>[2x]MGYLHRVVEGLKANAGGEALVSADRRLTGAETLEEIHRTARALAAQGLRPGDGVVTLHGNGVEAVVLRIAVQLLGCRYAGLRPVFATREKANFLAEAEAAAFVYQPDMADEAAELLREVPTPRVLSLGPAPLGEDLVALAGAQSAEPVEFTADERAATAVGFTGGTTGRAKGVCRAPFDLEACLDASLTIFGEGPWRFLVCIPIADLGGEMAEWTLAAGGTVVLREDFEPADILATIGAERTTHVFCAPGWVYQLAEHPALADADLSSLTQIPYGGAPSTPARIADALEKLGRPLLVHCYGSQEGGWMTWLSAEDHVRADRYLLNSVGKALPGTEIAIRDQDGADLPVGTVGEVCVRSTMLMRGYWRLPELTAKTVRDGWLHTGDLGRLDTEGYLYLVDRAKDVIIVEAYNVYSQEVEHVLTGHPDVRYAAVVGVPDHDTTEAVYAAVVPAEGVGEIDVDELRALVRTTLGPVHEPKHLDVVDTIPTTPRGHPDKSALRTRWRA

Amide Bond Synthetases (ABSs) actively catalyze both the ATP-dependent adenylation of carboxylic acid substrates and their subsequent amidation using an amine nucleophile, both within the active site of the enzyme, enabling the use of only a small excess of the amine partner. In this report, we describe the activity and specificity of an ABS from Streptoalloteichus hindustanus (ShABS), with a broader, complementary substrate spectrum to that of McbA that includes enantioselective behavior toward an expanded range of acid and amine partners in amidation reactions. The requirement for large excesses of amine in these reactions has prompted investigations into the ATP-dependent amide bond synthetase (ABS) class of enzymes, also members of the larger ANL (acyl-CoA synthetase–non-ribosomal peptide synthase–luciferase) family of adenylase enzymes, as these catalyze both the formation of the adenylate and the amidation reaction within one active site of the enzyme and require only one or low equivalents of the amine as a coupling partner. In common with other adenylases, McbA features a larger N-terminal domain coupled to a C-terminal “cap” domain.

As crystals of wild-type ShABS were initially not forthcoming, two mutants, K492A and K492H, of a lysine residue K492 implicated in interacting with ATP were prepared and subjected to crystallization trials, in an attempt to obtain a structure. Although no crystals were obtained in the presence of ATP or AMP and acid substrate, the inclusion of the noncleavable ATP analogue α,β-methylene adenosine 5′-triphosphate (AMP-CPP) was successful in giving diffracting crystals of ShABS K492H in the P21 space group, from which were obtained data sets that were refined to 2.01 (Data set #1) and 2.57 Ångstrom (Data set #2) resolution, the second of which contained density for AMP-CPP in the active site. This structure of ShABS (ShABSAdFigure 1a) featured two molecules in the asymmetric unit cell, each of which corresponded to the “adenylation” conformation of McbA, with an rmsd between the two enzymes of 1.50 Å over 469 C-α atoms. In the structure of ShABSAd obtained from Data set #1, following the building of the protein and water atoms, residual density in the omit maps was clearly visible, and this could be successfully modeled and refined as α,β-methylene adenosine 5′-triphosphate (AMP-CPP). Superimposition of ShABSAd and McbAAd permitted the positioning of the acid substrate 5 within the active site and a consequent analysis of probable active site interactions. The major differences in active site residues between the ShABSAd and McbAAd acid binding sites were W307 (ShABS) for F301 (McbA), W214 for C209, R175 for H170, C299 for N293, and S302 for T296. The presence of the two tryptophan residues is most likely to account for the differences in acid specificity between McbA and ShABS.>[2x]SMGKLSEHLRYCDSILREMLSKKHAAYAWPFYKPVDAEALELHDYHDI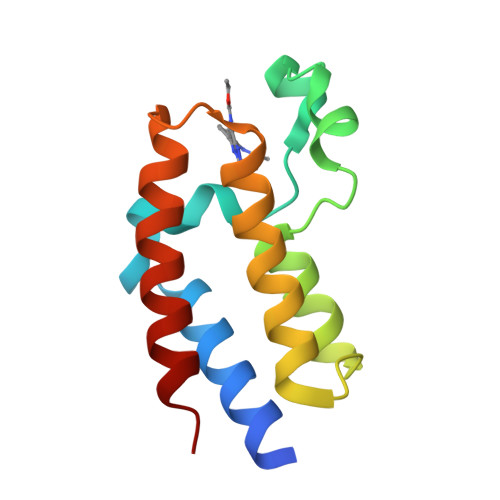IKHPMDLSTVKRKMDGREYPDAQGFAADVRLMFSNCYKYNPPDHEVVAMARKLQDVFEMRFAKMP N,N-dimethylpyridin-4-amine | C7 H10 N2 | 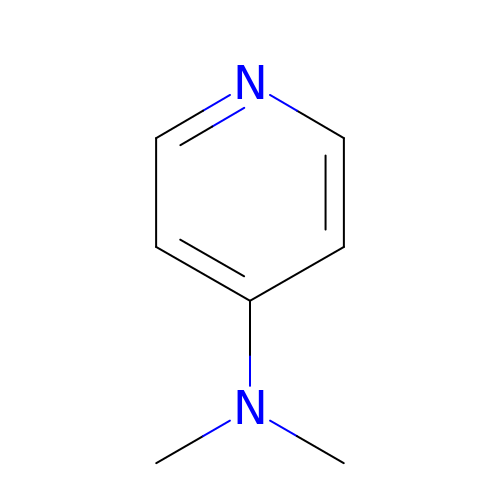VHYFNPMBLIVWCW-UHFFFAOYSA-N>[2x]MTNGDNLAQIGVVGLAVMGSNLARNFARNGNTVAVYNRSTDKTDKLIADHGSEGNFIPSATVEEFVASLEKPRRAIIMVQAGNATDAVINQLADAMDEGDIIIDGGNALYTDTIRREKEISARGLHFVGAGISGGEEGALNGPSIMPGGPAKSYESLGPLLESIAANVDGTPCVTHIGPDGAGHFVKMVHNGIEYADMQVIGEAYHLLRYAAGMQPAEIAEVFKEWNAGDLDSYLIEITAEVLSQVDAETGKPLIDVIVDAAGQKGTGRWTVKAALDLGIATTGIGEAVFARALSGATSQRAAAQGNLPAGVLTDLEALGVDKAQFVEDVRRALYASKLVAYAQGFDEIKAGSDENNWDVDPRDLATIWRGGCIIRAKFLNRIVEAYDANAELESLLLDPYFKSELGDLIDSWRRVIVTATQLGLPIPVFASSLSYYDSLRAERLPAALIQGQRDFFGAHTYKRIDKDGSFHTEWSGDRSEVEALEHHHHHH

In summary, we determined the crystal structures of the apo and complex forms of Cg6PGD with a resolution of 2.4 and 1.9 Å, respectively; Cg6PGD is the crucial enzyme in NADPH production. Cg6PGD eluted with a molecular weight of approximately 116.8 kDa, indicating that Cg6PGD exists as a dimer in solution. The monomeric structure of Cg6PGD could be divided into three functional domains : the N-terminal domain (N-term domain, Met1-Pro179), the central domain (CD, Asp180-Arg441), and the C-terminal domain (C-term domain, Ala442-Ala484). The CD consisted of α-helices exclusively and was associated with dimerization.

The crystal forms of both structures included a dimer per asymmetric unit. To characterize the conformational change between Cg6PGD_apo and Cg6PGD_NADP, we determined the crystal structures of both forms. Structural differences between Cg6PGD_apo and Cg6PGD_NADP were detected in the residual movement together with the loop. To predict the substrate-binding site of Cg6PGD, similar structures (Gs6PGD and Ec6PGD) were used to perform alignments, which revealed that the Asn107, Ser133, Gly134, Gly135, Lys187, Asn191, Glu194, Tyr195, Lys265, Thr267, Arg292, Arg454, and His460 residues were involved in the binding to substrate in Cg6PGD. In turn, the Tyr195, Lys265, Arg292 and Arg454 residues stabilized the phosphate moiety of 6PG through hydrogen bonds, and the Asn191, Glu194 and Thr267 residues also formed a water-mediated hydrogen bond with the phosphate moiety of 6PG. Docking simulations of the substrate were also performed to predict the substrate-binding mode. The 6PG molecule fitted the substrate-binding cavity well, which was predicted based on other similar structure. In the substrate-binding pocket, the N-term domain, CD, C-term domain were involved in the binding of substrate.> MLLREINRYCKEKATGKRIYAVPKLWIPGFFKKFDEKSGRCFVDPYELGAEITDWILNQSREWDYSQPLSFLKGEKTPDWIKRSVVYGSLPRTTAAYNHKGSGYYEENDVLGFREAGTFFKMML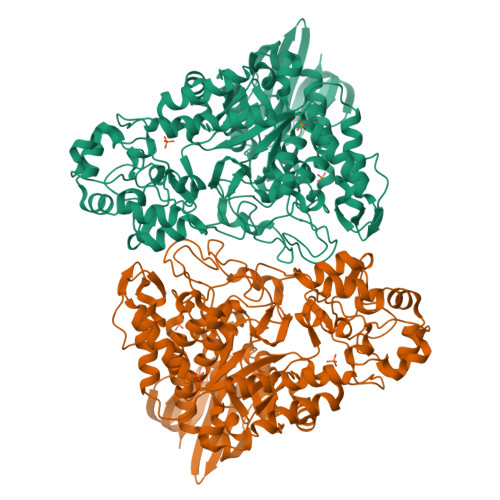LLPFVKSLGADAIYLLPVSRMSDLFKKGDAPSPYSVKNPMELDERYHDPLLEPFKVDEEFKAFVEACHILGIRVILDFIPRTAARDSDLIREHPDWFYWIKVEELADYTPPRAEELPFKVPDEDELEIIYNKENVKRHLKKFTLPPNLIDPQKWEKIKREEGNILELIVKEFGIITPPGFSDLINDPQPTWDDVTFLRLYLDHPEASKRFLDPNQPPYVLYDVIKASKFPGKEPNRELWEYLAGVIPHYQKKYGIDGARLDMGHALPKELLDLIIKNVKEYDPAFVMIAEELDMEKDKASKEAGYDVILGSSWYFAGRVEEIGKLPDIAEELVLPFLASVETPDTPRIATRKYASKMKKLAPFVTYFLPNSIPYVNTGQEIGEKQPMNLGLDTDPNLRKVLSPTDEFFGKLAFFDHYVLHWDSPDRGVLNFIKKLIKVRHEFLDFVLNGKFENLTTKDLVMYSYEKNGQKIVIAANVGKEPKEITGGRVWNGKWSDEEKVVLKPLEFALVVQE>[6x]MGSSPHHHHHSQDPMLSKDIIKLLNEQVNKEMNSSNLYMSMSSWCYTHSLDGAGL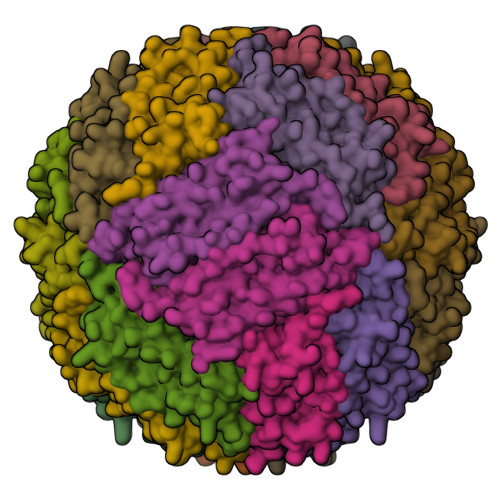FLFDHAAEEYEHAKKLIIFLNENNVPVQLTSISAPEHKFEGLTQIFQKAYEHEQHISESINNIVDHAIKSKDHATFNFLQWYVAEQHEEEVLFKDILDKIELIGNENHGLYLADQYVKGIAKSRKS> GSHMALDLTGYLDRINYRGATDPTLDVLRDLVSAHTGA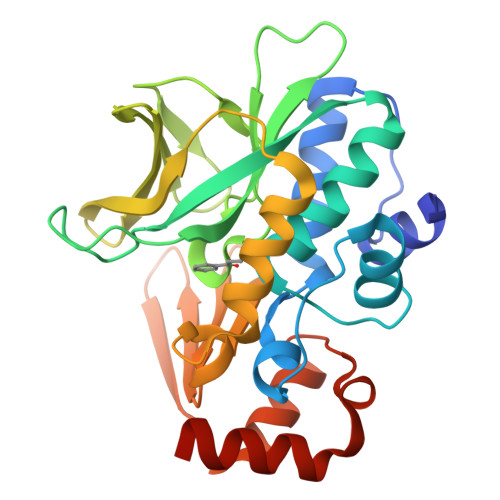IAFENLDPLMGVPVDDLSAEALADKLVDRRRGGYCYEHNGLIGYVLAELGYRVRRLAGRVVWLAPPDAPTPAQTHTVLAVTFPGCQGPYLVDVGFGGMTPTAPLRLETGTVQQTALEPYRLDDRGDGLVLQAMVRDEWQALYEFSTLTRPQVDLRVGSWFVSTHPTSHFVTGLMAATVADDARWNLMGRNLAIHRRGGTEKILLEDAAAVVDTLGDRFGINVADVGERGRLEARIDKVCFGAENR> MSVVTKSIVNADAEARYLSPGELDRIKNFVSTGERRLRIAQTLTENRERIVKQ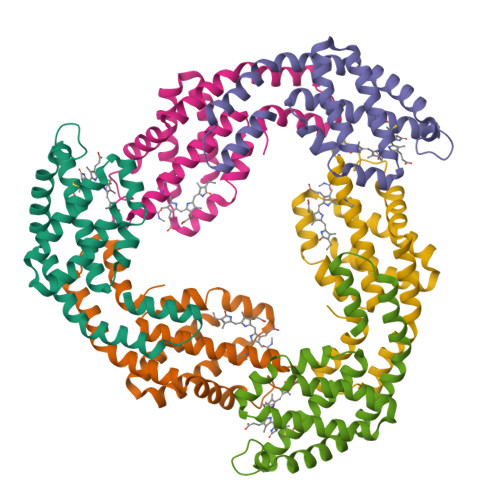AGDQLFQKRPDVVSPGGNAYGEEMTATCLRDLDYYLRLVTYGIVAGDVTPIEEIGLVGVREMYNSLGTPIPAVAEGIRAMKNVACSLLSAEDAAEAGSYFDFVIGAMQ;> MQDAITAVINASDVQGKYLDTAAMEKLKAYFATGELRVRAASVISANAANIVKEAVAKSLLYSDITRPGGNMYTTRRYAACIRDLDYYLRYATYAMLAGDPSILDERVLNGLKETYNSLGVPIAATVQAIQAMKEVTASLVGADAGKEMGIYFDYICSGLS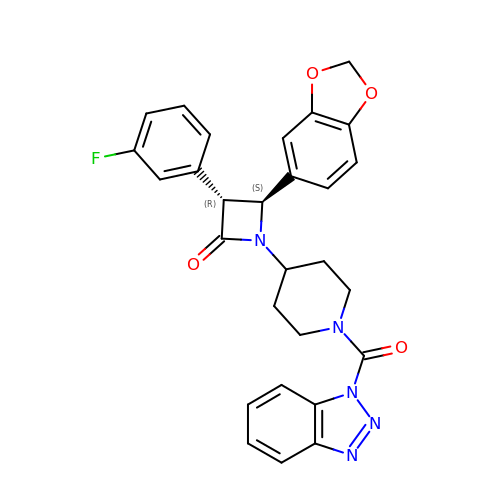(3~{R},4~{S})-4-(1,3-benzodioxol-5-yl)-1-[1-(benzotriazol-1-ylcarbonyl)piperidin-4-yl]-3-(3-fluorophenyl)azetidin-2-one | C28 H24 F N5 O4 | ZYBYLXKHKPMAIL-CLJLJLNGSA-N5-cyclohexyl-3-propyl-1H-pyridin-2-one 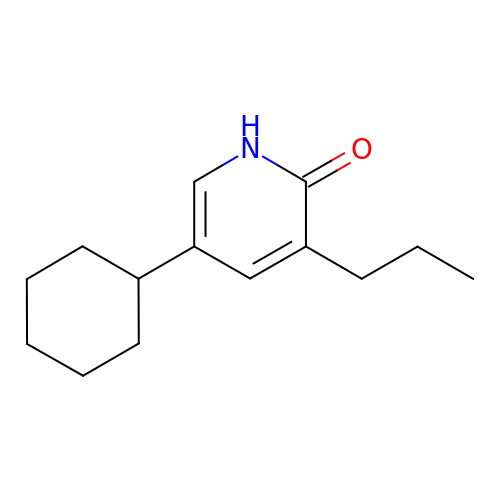| C14 H21 N O | VGWMLHHFTHSIBB-UHFFFAOYSA-N> VSDAVKKLRLPASMIIDGESPRFDDSIIPRHHGACFNVFIPAPPSHVPEVFTDRDITALIRAGGKDDELI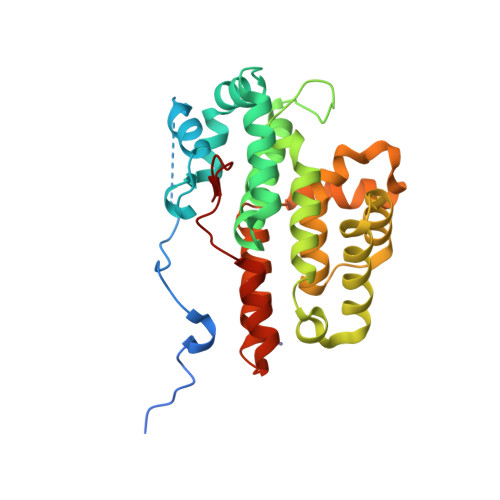NKKISAKKIDHLHRQMLSFVTSRHNQAYWVSCRRETAAAGGLQTLGAFVEEQMTWAQTVVRHGGWFDEKDIDIILDTAIFVCNAFVTRFRLLHLSCVFDKQSELALIKQVAYLVAMGNRLVEACNLLGEVKLNFRGGLLLAFVLTIPGMQSRRSISARGQELFRTLLEYYRPGDVMGLLNVIVMEHHSLCRNSECAAATRAAMGSAKFNKGLFFYPLS> QQDQ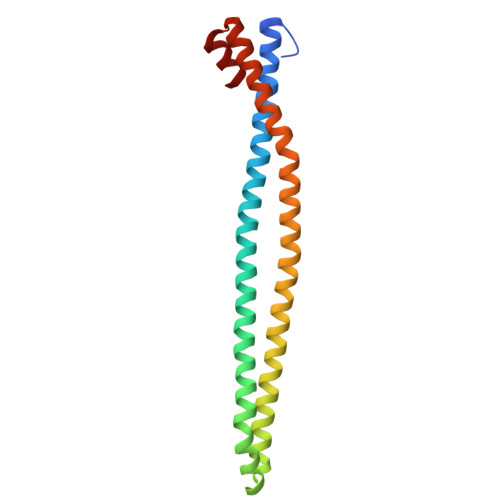VVKEDNIEAVGKKLHEYNTQFQEKSREYDRLYEDYTRTSQEIQMKRTAIEAFNETIKIFEEQCQTQERYSKEYIEKFKREGNETEIQRIMHNYEKLKSRISEIVDSRRRLEEDLKKQAAEYREIDKRMNSIKPDLIQLRKTRDQYLMWLTQKGVRQKKLNEWLG> MGSDKIHHHHHHMNVINETANVLKLETGSVTSAKGFSAVGIHTGVKRKRKDLGAIVCEVPASSAAVYTLNKVQ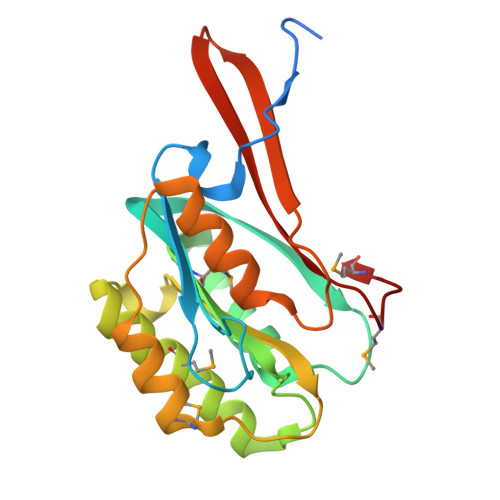AAPLKVTQESIAVEGKLQAMIVNSGIANACTGKRGLDDAYTMRAVGAETFHIPEHYVAVTSTGVIGEFLPMDVITNGIRQLKPEATIEGAHAFNEAILTTDTVEKHTCYQTIVNGKTVTVGGVAKGSGMIHPNMA> YKYKQKPKYQVRWKIIESYEGNSYTFIDPTQLPYNEKWEFPRNNLQFGKTLGAGAFGKVVEATAFGLGKEDAVLKVAVKMLKSTAHADEKEALMSELKIMSHLGQHE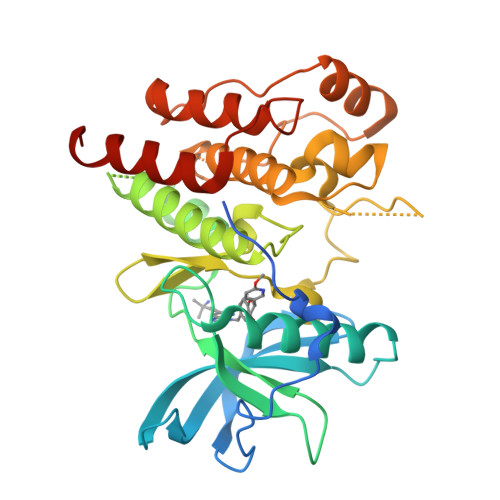NIVNLLGACTHGGPVLVITEYCCYGDLLNFLRRKSPPGLEYSYNPSHNPEEQLSSRDLLHFSSQVAQGMAFLASKNCIHRDVAARNVLLTNGHVAKIGDFGLARDIMNDSNYIVKGNARLPVKWMAPESIFDCVYTVQSDVWSYGILLWEIFSLGLNPYPGILVNSKFYKLVKDGYQMAQPAFAPKNIYSIMQACWALEPTHRPTFQQICSFLQEQAQEDRRERD>AIKVCMNALCGAASTSGEWKKGWPMRSGDLASLCDKCGCAYEQSIFCEVFHAKESGWRECNSCDKRLHCGCIASRFM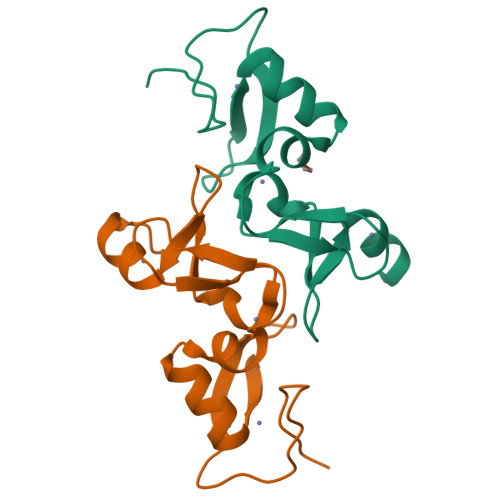MELLENGGVTCISCAKKSGLISMNVS[2x]8-[(6-IODO-1,3-BENZODIOXOL-5-YL)THIO]-9-[3-(ISOPROPYLAMINO)PROPYL]-9H-PURIN-6-AMINE | C18 H21 I N6 O2 S | 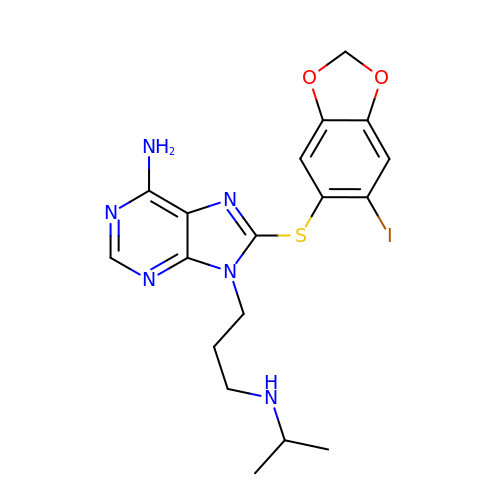SUPVGFZUWFMATN-UHFFFAOYSA-N>[4x]MIG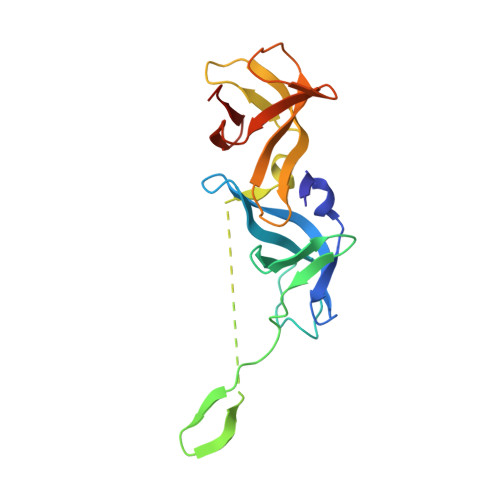EITTFFGMRVFTDEGRYVGRVEDVILDQNTKSIRGLAISDYNKALIDSHAKGVIIPYRVVKAVGDIIIIKDLFKRKSRVLDYESRELIEEEGEEGEEWQEMYVPARSLARKSVVLTDGTVVGTLYNITVDFKTGTIVNLLVKPENEIPDFKKEEGLYIIPFECVRSLKDFIVVDRRRVR>[2x]QIQIPASEQETLVRPKPLLLKLLKS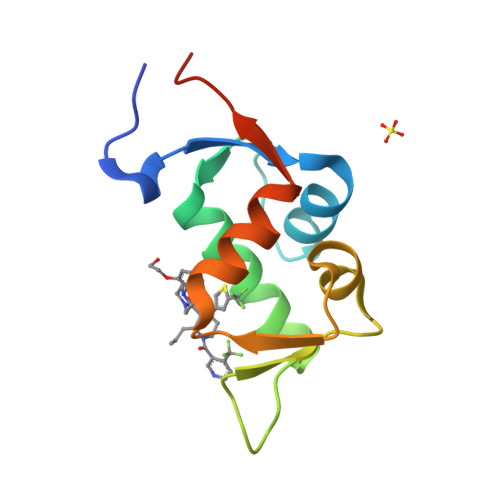VGAQKDTYTMKEVLYYLGQYIMTKRLYDEKQQHIVHCSNDLLGDLFGVPSFSVKEHRKIYTMIYRNLVVVNQQESSAGA>[2x]EDELYRQSLEIISRYLREQATGAKDTKPMGRSGA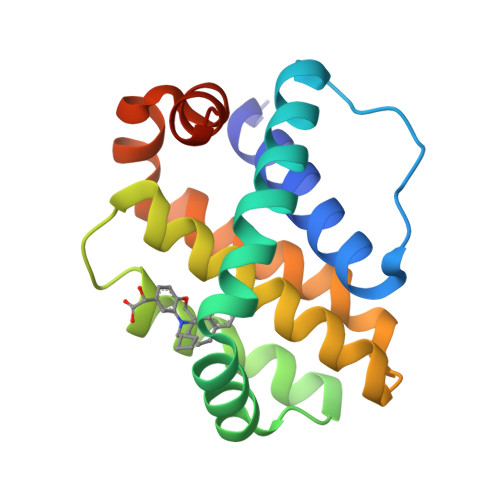TSRKALETLRRVGDGVQRNHETAFQGMLRKLDIKNEDDVKSLSRVMIHVFSDGVTNWGRIVTLISFGAFVAKHLKTINQESCIEPLAESITDVLVRTKRDWLVKQRGWDGFVEFFHVEDLEGG> MAKVRIYQLAKELGMETQELLELLDQMGVAYKSHASTLEEKDAEAVRELVKEQRGLQEKLAEEERRKSLPRRPPVVVIMGHVDHGKTTLLDYLRKSRIAEKEAGGITQHVGAFEVKTPQGTVVFIDTPGHEAFTTIRQRGAKVADIAVIVIAADDGIMPQTEEAIAHAKAAGAKLIFAINKIDLPQADPEKVKRQLMERGFVPEEYGGDAIVIPISAKTGQGVQDLLEMILLLAELEDYRADPNAEPRGVILESKLDKQAGIIANMLVQEGTFRVGDYVVAGEAYGRIRAMMDADGNQRKEAGPGSAVQVLGFQELPHAGDVVEWVPDLEAAKEIAEERKEERKAREEEEKARAPATMAALLAAMAEEGAKELNLILRADTQGSLEAIQHILARA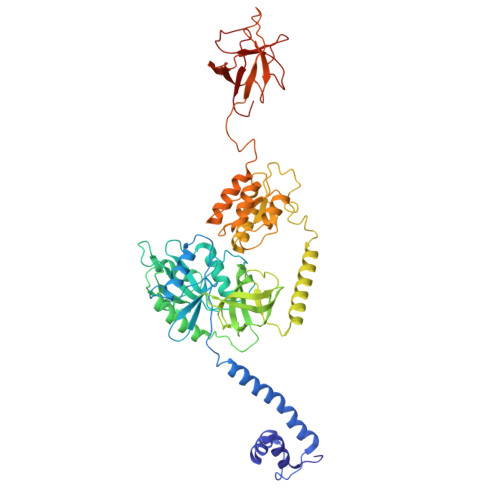TTEDVKINILAAQVGAPTESDVLLAQTANAAILAFGVNPPGSVKKKAEEKGVLLKTFRIIYDLVDEVRNMVKGAREPQYKEEVLGQAEVRAIFRLPTGKQVAGCMVTQGRIPRNAEVRVLRDGQVIWQGRIASLKRFKEDVREVAQGYECGIGLDGFDDFREGDVIEAFQMVEV>[4x]SMRVKAAQAGRQSSAKRHLAEQFAVGEIITDMAAAAWKVGLPIGQGGFGCIYLADMNSSESVGSDAPCVVKVEPSDNGPLFTELKFYQRAAKPEQIQKWIRTRKLKYLGVPKYWGSGLHDKNGKSYRFMIMDRFGSDLQKIYEANAKRFSRKTVLQLSLRILDILEYIHEHEY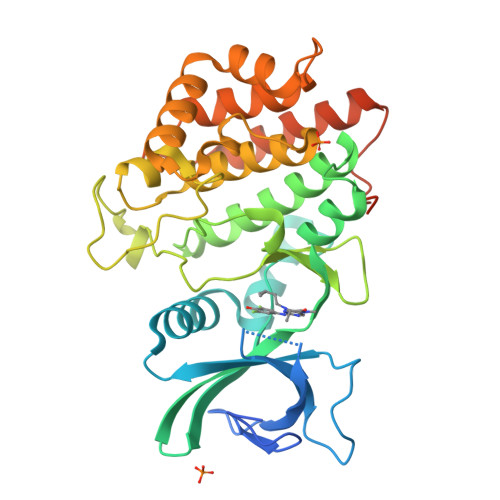VHGDIKASNLLLNYKNPDQVYLVDYGLAYRYCPEGVHKAYAADPKRCHDGTIEFTSIDAHNGVAPSRRGDLEILGYCMIQWLTGHLPWEDNLKDPKYVRDSKIRYRENIASLMDKCFPAANAPGEIAKYMETVKLLDYTEKPLYENLRDILLQGLKAIGSKDDGKLDLSVVENGGLKAKTITKKRAAEIEE The localization of motility complexes, and thereby the direction of movement, is determined by an oscillatory system, which includes Mutual gliding motility A (MglA), a small Ras-like GTPase, and Mutual gliding motility B (MglB), its GTPase activating protein (GAP) as major components. In this study, we report the biochemical and structural characterization of M. xanthus MglA and MglB (MxMglA and MxMglB). Thus, MxMglB plays a dual role in increasing the GTPase activity of MxMglA by orienting the catalytic residues (role of a GAP) and by facilitating exchange of GDP with GTP (role of a GEF). Allosteric binding of the C-terminal helix (Ct-helix) of MxMglB on MxMglA facilitates nucleotide exchange.

Structure of MxMglA is similar to TtMglA with 2 additional β-strands (β0 and β2*), compared with the 5 α-helices and 6 β-strands present in the small Ras-like GTPase fold. All the residues of the small Ras-like GTPase fold as well as the C-terminal hexahistidine tag were modeled in the MxMglA structure. Though GDP was not added during protein purification or crystallization, the crystal structure of MxMglA contained GDP in the nucleotide-binding pocket. High-performance liquid chromatography (HPLC) analysis of the protein sample reconfirmed that the bound ligand is GDP. The purified MxMglA contained GDP bound to the active site pocket.

>MSFINYSSREINCKIVYYGPGLCGKTTNLQYIYNKTAAETKGKLISLSTETDRTLFFDFLPLSLGEIRGFKTRFHLYTVPGQVFYDASRKLILKGVDGVVFVADSQIERMEANMESLENLRINLAEQGYDLNKIPYVIQYNKRDLPNAVTVEEMRKALNHRNIPEYQAVAPTGVGVFDTLKAVAKLVLTELKKGGGSHHHHHH[2x]The conserved shelterin complex caps chromosome ends to protect telomeres and regulate telomere replication. In fission yeast Schizosaccharomyces pombe, shelterin consists of telomeric single- and double-stranded DNA-binding modules Pot1-Tpz1 and Taz1-Rap1 connected by Poz1, and a specific component Ccq1. Here, we report the crystal structures of Pot1DBD-single-stranded-DNA, Pot1372-555-Tpz1185-212 and Tpz1425-470-Ccq1123-439 complexes and propose an integrated model depicting the assembly mechanism of the shelterin complex at telomeres. Overall, our findings provide valuable structural information regarding interactions within fission yeast shelterin complex at 3’ ss telomeric overhang.

Consistent with previous Co-IP data, our biochemical analysis using purified proteins showed that a short and highly conserved fragment of Tpz1 (residues 185–212) is sufficient to maintain a stable interaction with Pot1372-555. We crystallized the Pot1372-555-Tpz1PIM complex and determined its structure by single-wavelength anomalous dispersion (SAD) method at a resolution of 2.6 Å. The crystal structure reveals that Pot1372-555 adopts a typical OB-fold architecture containing a highly curved five-stranded β-barrel, hereafter referred to as Pot1OB3. In the Pot1OB3-Tpz1PIM complex, the Tpz1PIM polypeptide exhibits an extended conformation with three separated helices (H1, H2 and H3). Helices H1 and H2 of Tpz1PIM lie in a continuous groove on the concaved side of the Pot1OB3, whereas helix H3 sits on a positively charged surface on the other side of Pot1OB3. The formation of the binary complex buries a total of ~1,200 Å2 solvent exposed surface area at the interface. The N-terminal 310 helix H1 of Tpz1PIM and its peripheral residues fit into a hydrophobic depression formed by strands β1, β2 and β3 of Pot1OB3. The short H2 helix fits into a narrow cleft formed by a two-stranded β1’- β2 protrusion and the long loop between strands β4 and β5 of Pot1OB3, with the sidechain of Cys198 pointing into the deep hydrophobic groove. In contrast to helices H1 and H2, helix H3 and its peripheral residues are away from the major binding groove of Pot1OB3, attaching to a rather flat surface of Pot1OB3 formed by strands β1, β4, and β5 through both electrostatic and hydrophobic contacts. Consistent with the crystal structure, single amino-acid substitution of Pot1-Leu441, Pot1-pro451, Pot1-Ile453 or Tpz1-Leu193 at the H1-binding interface, or Tpz1-Cys198, Tpz1-Ile200 or Tpz1-Pro201 at the H2-binding interface with positively charged arginine residue completely abolished the interaction between Pot1OB3 and Tpz1PIM.

>SENPFIAHELKQTSVNEITAHVINEPASLKLTTISTILHAPLQNLLKPRKHRLRVQVVDFWPKSLTQFAVLSQPPSSYVWMFALLVRDVSNVTLPVIFFDSDAAELINSSKIQPCNLADHPQMTLQLKERLFLIWGNLEERIQHHISKGESPTLAAEDVETPWFDIYVKEYIPVIGNTKDHQSLTFLQKRWRGFGTKIV[2x];>[2x]SQQEKPNDNTSNSRDIKNNIQFHWKNMTSLSIEECIIPKGQQLILEKESEENTTHGIYLEERKMAQGLHNSVSETPE>SRCTHLENRDFVTGTQGTTRVTLVLELGGCVTITAEGKPSMDVWLDAIYQENPAKTREYCLHAKLSDTKVAARCPTMGPATLAEEHQGGTVCKRDQSDRGHGNHCGLFGKGSIVACVKAACEAKKKATGHVYDANKIVYTVKVEPHTGDYVAANETHSGRKTASFTISSEKTILTMGEYGDVSLLCRVASGVDLAQTVILELDKTVEHLPTAWQVHRDWFNDLALPWKHEGAQNWNNAERLVEFGAPHAVKMDVYNLGDQTGVLLKALAGVPVAHIEGTKYHLKSGHVTCEVGLEKLKMKGLTYTMCDKTKFTWKRAPTDSGHDTVVMEVTFSGTKPCRIPVRAVAHGSPDVNVAMLITPNPTIENNGGGFIEMQLPPGDNIIYVGELSHQWFQKGSSIGRVFQGGGSGGGSGGFLSSIGKAVHTVLGGAFNSIGPFEDDDDKAGWSHPQFEK[3x]

Flaviviruses enter cells by fusion with endosomal membranes through a rearrangement of the envelope protein E, a class II membrane fusion protein, into fusogenic trimers. The rod‐like E subunits bend into “hairpins” to bring the fusion loops next to the C‐terminal transmembrane (TM) anchors, with the TM‐proximal “stem” element zippering the E trimer to force apposition of the membranes. The E protein is about 500 amino acids (aa) long, with an ectodomain formed by the ~ 400 N‐terminal aa and folded as three β‐sheet rich domains I, II, and III. The ectodomain is followed by a flexible region termed “stem” that tethers it to the C‐terminal transmembrane (TM) helices.

19, which suggested a role for sequence elements in the distal stem in zippering, we designed a recombinant soluble TBEV E protein (sE‐linker) in which an 8‐residue linker (GGGSGGGS) connected Gln404 to Gly427 and the following H3, bypassing most of the proximal stem, i.e., the second half of H1, H2, and the CS. We also introduced the same mutation in the FL (W101H) described in the DENV1 work 19 into the sE‐linker construct (sE‐linker* mutant), to enhance solubility and facilitate trimerization at low pH under crystallization conditions in the absence of detergent. We obtained crystals of the rhombohedral space group H3 diffracting to 2.6 Å resolution. The crystals displayed clear electron density except for the region of the tip of domain II, including the bcd β‐sheet (bearing the FL in the cd loop) and the ij β‐hairpin, which were not resolved. Nevertheless, the density was clear for the stem up to the last residue before the linker (Gln404), which corresponds to Glu403 in DENV1 E —the last residue resolved in that structure 19. As in the DENV1 sE trimer, in the TBEV sE‐linker* structure the stem adopts an extended conformation running within a groove, termed the “αA/B” groove, at the inner surface of domain II of the same chain, formed in between α‐helices A and B and bounded by the 3/10 helical turn η3 (see Appendix Fig S1 for the secondary structure nomenclature). The stem side chains alternate between inter‐ and intra‐chain contacts: those of Ser397, Ile399, Val402, and Gln404 interact with the adjacent subunit, whereas Ser398, Arg401, and Phe403 interact with domain II of the same protomer (the register change from odd to even residues is caused by a bulge of the main chain at Gly400). The domain II region involved in inter‐chain contacts with the stem includes the aa 230–238 region between β‐strand h and helix η3 preceding the ij β‐hairpin, with the Gln404 side chain hydrogen bonding the main chain of the neighboring subunit at residue 233. The only differences are due to a three‐residue insertion in DENV1 E in the βh‐η3 loop, which makes additional contacts and creates a narrower path for the stem.>RPQYRILGQIPDTDIYCDVEEYEEVKEYPGIKIFQANTSLYFANSESYTSALKKKTGVDGSTNVHSLILDFAPVNFVDSVGAKTLKSVIKEYNEVGVCVCIASCSGPVMNELTRLNFFDNTVTRE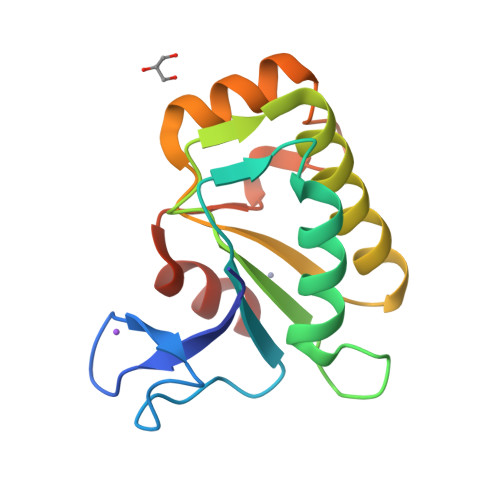LLFHSIHDAVLACQGKDR[2x]> MHHHHHHMVEVKKHKFPGVYVVIDDDGSEKIATKNLVPGQRVYGERVIKWEGEEYRIWNPHRSKLG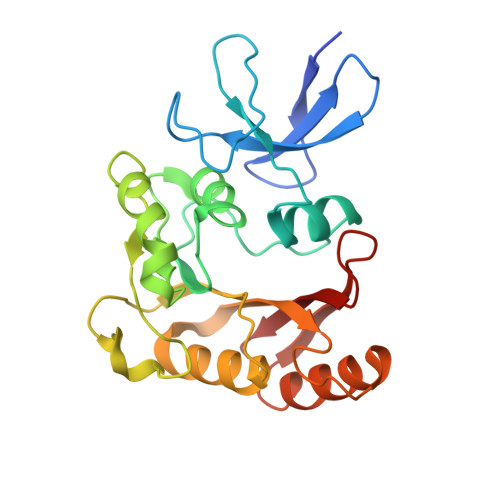AAIVNGLKNFPIKPGKSVLYLGIASGTTASHVSDIVGWEGKIYGIEFSPRVLRELVPIVEERRNIIPILGDATKPEEYRALVTKVDVIFEDVAQPTQAKILIDNAKAYLKRGGYGMIAVKSRSIDVTKEPEQVFKEVERELSEYFEVIERLNLEPYEKDHALFVVRKP> SRERIVPVVYYLSRNGRLDHPHFIEVPLSSHNGLYLKDVINRLNDLRGNGMACLYSWSSKRTYKNGFVWYALSDEDFIFPVH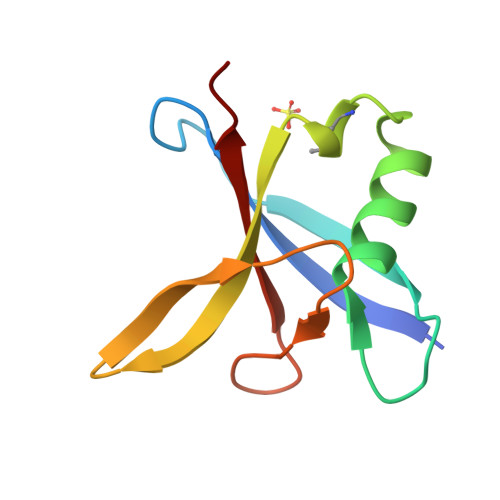GQEYVLKGSQILD> XEVKQLEAEVEEIESEVWHLENEV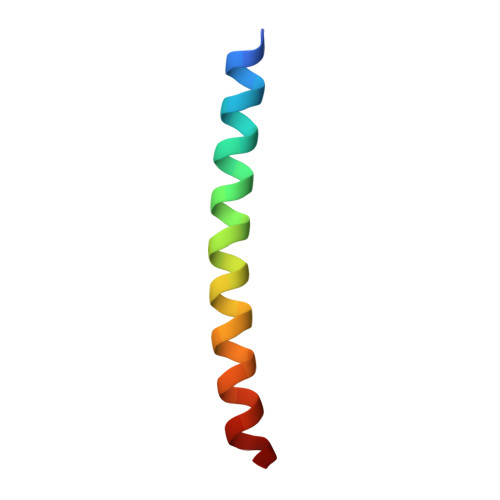ARLEKENAECEA>[4x]MGSSHHHHHHSSRNLYFQGGGHMFFLNLKQINDRFNTEFITKFKEILESGWYILGKQCEKFENNFAKYCGVKHCIGVANGLDALRLIIKAYDFKENDEIIVPANTYIASILAITDNKCKPILIEPDINTYNINPDLIEEKITKKTKAIMVVHLYGQVCDMEKIQLLANKYNLKIIEDCAQAHGAIYK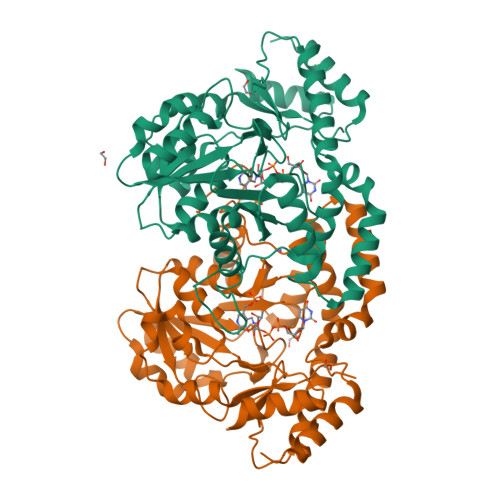DKRVGNLGDAAGFSFYPGANLGALGDAGCICTNDDNFASKIRALANYGSHKKYENLYTGLNSRLDEIQAAFLDIKLKYLDEDNNKRKNIANFYLQNIKNENIILPSNKFDHVWHLFVVKTKLRDELQHYLNNHDIQTIIHYPIPPHKQKCYKDLNHLKLPITENIHQEVLSLPISPTMKENDFKKVADILNKWKV> MEDLCVANTLFALNLFKHLAKASPTQNLFLSPWSISSTMAMVYMGSRGSTEDQMAKVLQFNEVGAAADKIHSSFRSLSSAINASTGNYLLESVNKLFGEKSASFREEYIRLCQKYYSSEPQAVDFLECAEEARKKINSWVKTQTKGKIPNLLPEGSVDGDTRMVLVNAVYFKGKWKTPFEKKLNGLYPFRVNSAQRTPVQMMYLREKLNIGYIEDLKAQILELPYAGDVSMFLLLPDEIADVSTGLELLESEITYDKLNKWTSKDKMAEDEVEVYIPQFKLEEHYELRSILRSMGMEDAFNKGRANFSGMSERNDLFLSEVFHQAMVD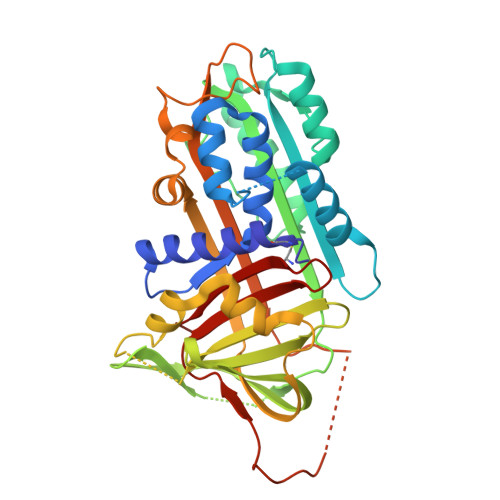VNEEGTEAAAGTGGVMTGRTGHGGPQFVADHPFLFLIMHKITNCILFFGRFSSP2-mercapto(3H)quinazolinone | C8 H6 N2 O S | 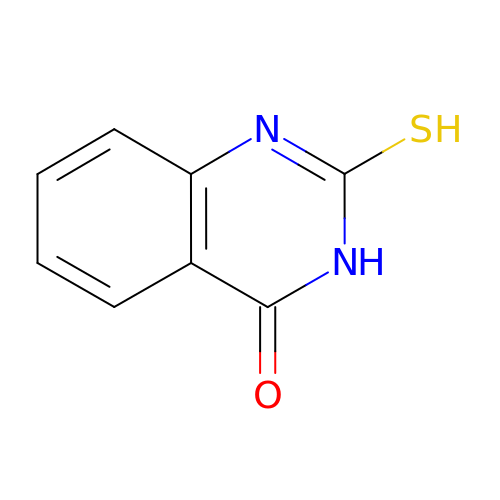PUPFOFVEHDNUJU-UHFFFAOYSA-N>SGQEFWPGQSAADILSGAASRRRYLLYDVNPPEGFNLRRDVYIRIASLLKTLLKTEEWVLVLPPWGRLYHWQSPDIHQVRIPWSEFFDLPSLNKNIPVIEYEQFIAESGGPFIDQVYVLQSYAEGWKEGTWEEKVDERPCIDQLLYSQDKHEYYRGWFWGYEETRGLNVSCLSVQGSASIVAPLLLRNTSARSVMLDRAENLLHDHYGGKEYWDTRRSMVFARHLREVGDEFRSRHLNSTDDADRIPFQEDWMKMKVKLGSALGGPYLGVHLRRKDFIWGHRQDVPSLEGAVRKIRSLMKTHRLDKVFVATDAVRKEYEELKKLLPEMVRFEPTWEELELYKDGGVAIIDQWICAHARFFIGTSVSTFS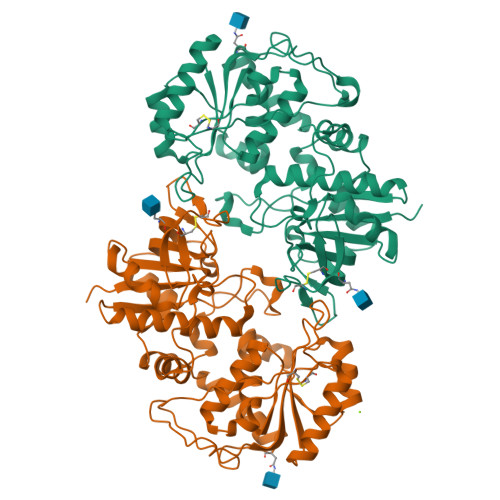FRIHEEREILGLDPKTTYNRFCGDQEKACEQPTHWKITY[2x]>HTVELNNMFGQIQSPGYPDSYPSDSEVTWNITVPDGFRIKLYFMHFNLESSYLCEYDYVKVETEDQVLATFCGRETTDTEQTPGQEVVLSPGSFMSITFRSDFSNE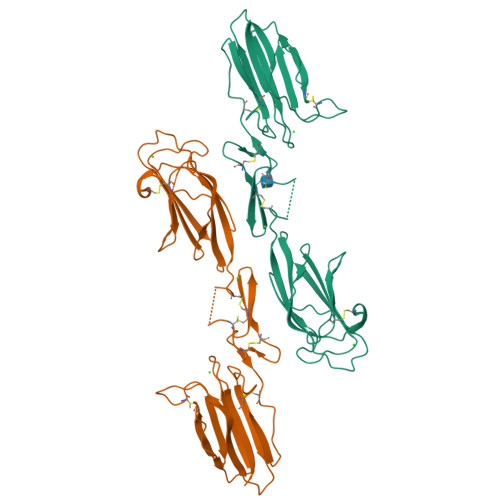ERFTGFDAHYMAVDVDECKEREDEELSCDHYCHNYIGGYYCSCRFGYILHTDNRTCRVECSDNLFTQRTGVITSPDFPNPYPKSSECLYTIELEEGFMVNLQFEDIFDIEDHPEVPCPYDYIKIKVGPKVLGPFCGEKAPEPISTQSHSVLILFHSDNSGENRGWRLSYRAA[2x]> GSHMSREEIRKVVEEYIRLLYTDPDQFKKAARDKLLSPDVRIEIGNYTFDSRNLDRFLDAMQEWASRYDRVEIRKVQVDGNHVRVEIELESNGKKWTFEIEVEVRNGKIKRIRQQVDPEYKKVVQNLWNN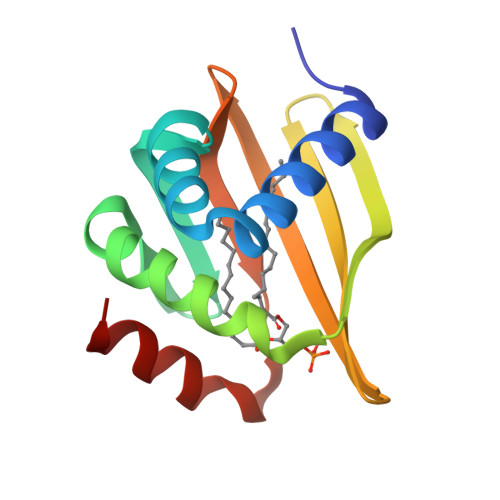T> GGACGAGGAGCGUUGCAAGCGAAAGCCCAGGCUAGUCCGUUCAAACGGCGCU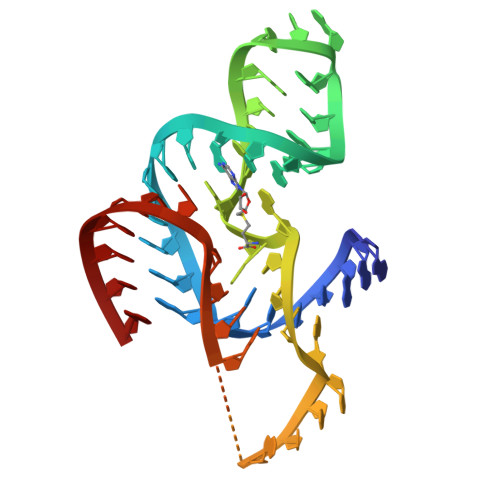CA> MPYSVGFREADAATSFLRAARSGNLDKALDHLRNGVDINTCNQNGLNGLHLASKEGHVKMVVELLHKEIILETTTKKGNTALHIAALAGQDEVVRELVNYGANVNAQSQKGFTPLYMAAQENHLEVVKFLLENGANQNVATEDGFTPLAVALQQGHENVVAHLINYGTKGKVRLPALHIAARNDDTRTAAVLLQNDPNPDVLSKTGFTPLHIAAHYENLNVAQLLLNRGASVNFTPQNGITPLHIASRRGNVIMVRLLLDRGAQIETKTKDELTPLHCAARNGHVRISEILLDHGAPIQAKTKNGLSPIHMAAQGDHLDCVRLLLQYDAEIDDITLDHLTPLHVAAHCGHHRVAKVLLDKGAKPNSRALNGFTPLHIACKKNHVRVMELLLKTGASIDAVTESGLTPLHVASFMGHLPIVKNLLQRGASPNVSNVKVETPLHMAARAGHTEVAKYLLQNKAKVNAKAKDDQTPLHCAARIGHTNMVKLLLENNANPNLATTAGHTPLHIAAREGHVETVLALLEKEASQACMTKKGFTPLHVAAKYGKVRVAELLLERDAHPNAAGKNGLTPLHVAVHHNNLDIVKLLLPRGGSPHSPAWNGYTPLHIAAKQNQVEVARSLLQYGGSANAESVQGVTPLHLAAQEGHAEMVALLLSKQANGNLGNKSGLTPLHLVAQEGHVPVADVLIKHGVMVDATTRMGYTPLHVASHYGNIKLVKFLLQHQADVNAKTKLGYSPLHQAAQQGHTDIVTLLLKNGASPNEVSSDGTTPLAIAKRLGYISVTDVLKVVTDETSFVLVSDKHRMSFPETVDEILDVSEDEGEELISFKAERRDSRDVDEEKELLDFVPKLDQVVESPAIPRIPCAMPETVVIRSEEQEQASKEYDEDSLIPSSPATETSDNISPVASPVHTGFLVSFMVDARGGSMRGSRHNGLRVVIPPRTCAAPTRITCRLVKPQKLSTPPPLAEEEGLASRIIALGPTGAQFLSPVIVEIPHFASHGRGDRELVVLRSENGSVWKEHRSRYGESYLDQILNGMDEELGSLEELEKKRVCRIITTDFPLYFVIMSRLCQDYDTIGPEGGSLKSKLVPLVQATFPENAVTKRVKLALQAQPVPDELVTKLLGNQATFSPIVTVEPRRRKFHRPIGLRIPLPPSWTDNPRDSGEGDTTSLRLLCSVIGGTDQAQWEDITGTTKLVYANECANFTTNVSARFWLSDCPRTAEAVNFATLLYKELTAVPYMAKFVIFAKMNDPREGRLRCYCMTDDKVDKTLEQHENFVEVARSRDIEVLEGMSLFAELSGNLVPVKKAAQQRSFHFQSFRENRLAMPVKVRDSSREPGGSLSFLRKAMKYEDTQHILCHLNITMPPCAKGSGAEDRRRTPTPLALRYSILSESTPGSLSGTEQAEMKMAVISEHLGLSWAELARELQFSVEDINRIRVENPNSLLEQSVALLNLWVIREGQNANMENLYTALQSIDRGEIVNMLEGSGRQSRNLKPDRRHTDRDYSLSPSQMNGYSSLQDELLSPASLGCALSSPLRADQYWNEVAVLDAIPLAATEHDTMLEMSDMQVWSAGLTPSLVTAEDSSLECSKAEDSDATGHEWKLEGALSEEPRGPELGSLELVEDDTVDSDATNGLIDLLEQEEGQRSEEKLPGSKRQDDATGAGQDSENEVSLVSGHQRGQARITHSPTVSQVTERSQDRLQDWDADGSIVSYLQDAAQGSWQEEVTQGPHSFQGTSTMTEGLEPGGSQEYEKVLVSVSEHTWTEQPEAESSQADRDRRQQGQEEQVQEAKNTFTQVVQGNEFQNIPGEQVTEEQFTDEQGNIVTKKIIRKVVRQIDLSSADAAQEHEEVTVEGPLEDPSELEVDIDYFMKHSKDHTSTPNP;>[2x]MYGKIIFVLLLSEIVSISASSTTGVAMHTSTSSSVTKSYISSQTNDTHKRDTYAATPRAHEVSEISVRTVYPPEEETGERVQLAHHFSEPEITLIIFGVMAGVIGTILLISYGIRRLIKKSPSDVKPLPSPDTDVPLSSVEIENPETSDQ;> MSSKYPRSVRRCLPLWALTLEAALILLFYFFTHYDASLEDQKGLVASYQVGQDLTVMAALGLGFLTSNFRRHSWSSVAFNLFMLALGVQWAILLDGFLSQFPPGKVVITLFSIRLATMSAMSVLISAGAVLGKVNLAQLVVMVLVEVTALGTLRMVISNIFNTDYHMNLRHFYVFAAYFGLTVAWCLPKPLPKGTEDNDQRATIPSLSAMLGALFLWMFWPSVNSPLLRSPIQRKNAMFNTYYALAVSVVTAISGSSLAHPQRKISMTYVHSAVLAGGVAVGTSCHLIPSPWLAMVLGLVAGLISIGGAKCLPVCCNRVLGIHHISVMHSIFSLLGLLGEITYIVLLVLHTVWNGNGMIGFQVLLSIGELSLAIVIALTSGLLTGLLLNLKIWKAPHVAKYFDDQVFWKFPHLAVGF;>MRFTFPLMAIVLEIAMIVLFGLFVEYETDQTVLEQLNITKPTDMGIFFELYPLFQDVHVMIFVGFGFLMTFLKKYGFSSVGINLLVAALGLQWGTIVQGILQSQGQKFNIGIKNMINADFSAATVLISFGAVLGKTSPTQ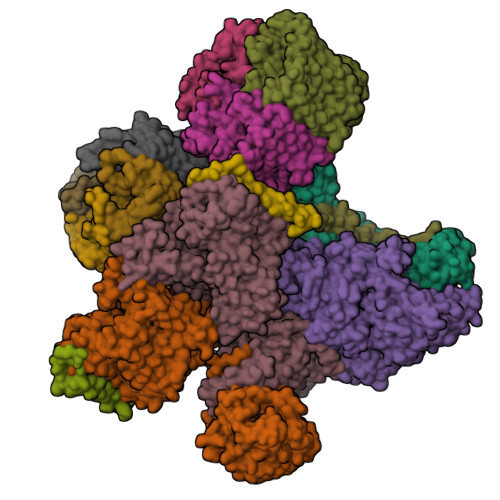MLIMTILEIVFFAHNEYLVSEIFKASDIGASMTIHAFGAYFGLAVAGILYRSGLRKGHENEESAYYSDLFAMIGTLFLWMFWPSFNSAIAEPGDKQCRAIVNTYFSLAACVLTAFAFSSLVEHRGKLNMVHIQNATLAGGVAVGTCADMAIHPFGSMIIGSIAGMVSVLGYKFLTPLFTTKLRIHDTCGVHNLHGLPGVVGGLAGIVAVAMGASNTSMAMQAAALGSSIGTAVVGGLMTGLILKLPLWGQPSDQNCYDDSVYWKVPKTR[2x];>[4x]MASEFKKKLFWRAVVAEFLATTLFVFISIGSALGFKYPVGNNQTAVQDNVKVSLAFGLSIATLAQSVGHISGAHLNPAVTLGLLLSCQISIFRALMYIIAQCVGAIVATAILSGITSSLTGNSLGRNDLADGVNSGQGLGIEIIGTLQLVLCVLATTDRRRRDLGGSAPLAIGLSVALGHLLAIDYTGCGINPARSFGSAVITHNFSNHWIFWVGPFIGGALAVLIYDFILAPRSSDLTDRVKVWTSGQVEEYDLDADDINSRVEMKPK;>MEELQDDYEDMMEENLEQEEYEDPDIPESQMEEPAAHDTEATATDYHTTSHPGTHKVYVELQELVMDEKNQELRWMEAARWVQLEENLGENGAWGRPHLSHLTFWSLLELRRVFTKGTVLLDLQETSLAGVANQLLDRFIFEDQIRPQDREELLRALLLKHSHAGELEALGGVKPAVLTRSGDPSQPLLPQHSSLETQLFCEQGDGGTEGHSPSGILEKIPPDSEATLVLVGRADFLEQPVLGFVRLQEAAELEAVELPVPIRFLFVLLGPEAPHIDYTQLGRAAATLMSERVFRIDAYMAQSRGELLHSLEGFLDCSLVLPPTDAPSEQALLSLVPVQRELLRRRYQSSPAKPDSSFYKGLDLNGGPDDPLQQTGQLFGGLVRDIRRRYPYYLSDITDAFSPQVLAAVIFIYFAALSPAITFGGLLGEKTRNQMGVSELLISTAVQGILFALLGAQPLLVVGFSGPLLVFEEAFFSFCETNGLEYIVGRVWIGFWLILLVVLVVAFEGSFLVRFISRYTQEIFSFLISLIFIYETFSKLIKIFQDHPLQKTYNYNVLMVPKPQGPLPNTALLSLVLMAGTFFFAMMLRKFKNSSYFPGKLRRVIGDFGVPISILIMVLVDFFIQDTYTQKLSVPDGFKVSNSSARGWVIHPLGLRSEFPIWMMFASALPALLVFILIFLESQITTLIVSKPERKMVKGSGFHLDLLLVVGMGGVAALFGMPWLSATTVRSVTHANALTVMGKASTPGAAAQIQEVKEQRISGLLVAVLVGLSILMEPILSRIPLAVLFGIFLYMGVTSLSGIQLFDRILLLFKPPKYHPDVPYVKRVKTWRMHLFTGIQIICLAVLWVVKSTPASLALPFVLILTVPLRRVLLPLIFRNVELQCLDADDAKATFDEEEGRDEYDEVAMPV[3x];> MGQALGIKSCDFQAARNNEEHHTKALSSRRLFVRRGQPFTIILYFRAPVRAFLPALKKVALTAQTGEQPSKINRTQATFPISSLGDRKWWSAVVEERDAQSWTISVTTPADAVIGHYSLLLQVSGRKQLLLGQFTLLFNPWNREDAVFLKNEAQRMEYLLNQNGLIYLGTADCIQAESWDFGQFEGDVIDLSLRLLSKDKQVEKWSQPVHVARVLGALLHFLKEQRVLPTPQTQATQEGALLNKRRGSVPILRQWLTGRGRPVYDGQAWVLAAVACTVLRCLGIPARVVTTFASAQGTGGRLLIDEYYNEEGLQNGEGQRGRIWIFQTSTECWMTRPALPQGYDGWQILHPSAPNGGGVLGSCDLVPVRAVKEGTLGLTPAVSDLFAAINASCVVWKCCEDGTLELTDSNTKYVGNNISTKGVGSDRCEDITQNYKYPEGSLQEKEVLERVEKEKMEREKDNGIRPPSLETASPLYLLLKAPSSLPLRGDAQISVTLVNHSEQEKAVQLAIGVQAVHYNGVLAAKLWRKKLHLTLSANLEKIITIGLFFSNFERNPPENTFLRLTAMATHSESNLSCFAQEDIAICRPHLAIKMPEKAEQYQPLTASVSLQNSLDAPMEDCVISILGRGLIHRERSYRFRSVWPENTMCAKFQFTPTHVGLQRLTVEVDCNMFQNLTNYKSVTVVAPELSA> 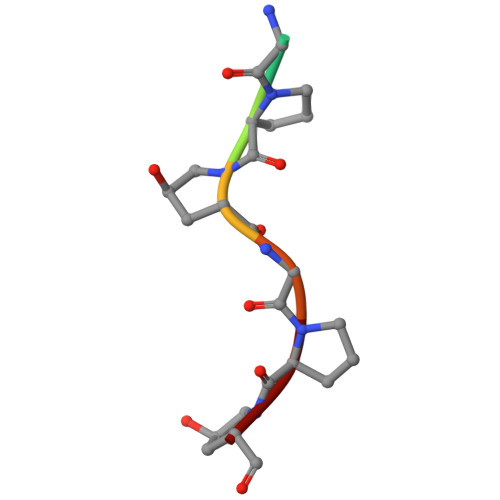PGPPGPP>MKYDLIIIGSGSVGAAAGYYATRAGLNVLMTDAHMPPHQHGSHHGDTRLIRHAYGEGEKYVPLVLRAQMLWDELSRHNEDDPIFVRSGVINLGPADSTFLANVAHSAEQWQLNVEKLDAQGIMARWPEIRVPDNYIGLFETDSGFLRSELAIKTWIQLAKEAGCAQLFNCPVTAIRHDDDGVTIETADGEYQAKKAIVCAGTWVKDLLPELPVQPVRKVFAWYQADGRYSVKNKFPAFTGELPNGDQYYGFPAENDALKIGKHNGGQVIHSADERVPFAEV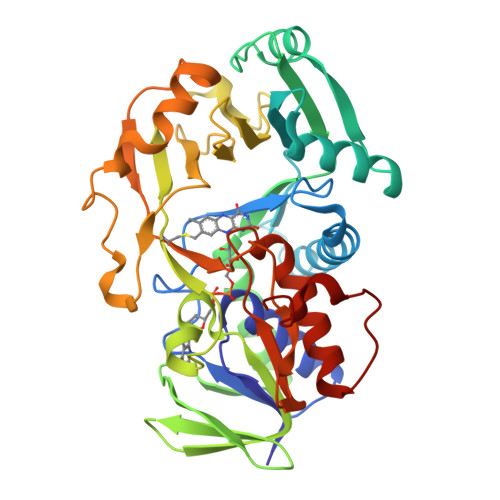VSDGSEAFPFLRNVLPGIGCCLYGAACTYDNSPDEDFIIDTLPGHDNTLLITGLSGHGFKFASVLGEIAADFAQDKKSDFDLTPFRLSRFQ[4x]>EEVRQFRRLFAQLAGDDMEVSATELMNILNKVVTRHPDLKTDGFGIDTCRSMVAVMDSDTTGKLGFEEFKYLWNNIKRWQAIYKQFDTDRSGTICSSELPGAFEAAGFHLNEHLYNMIIRRYSDESGNMDFDNFISCLVRLDAMFRAFKSLDKDGTGQIQVNIQEWLQLTMYS[2x]

Calpain-I and calpain-II are the two most studied members of a family of calcium dependent cysteine proteases that currently comprises fifteen identified gene products in humans. These heterodimeric proteases are composed of a large subunit with a molecular mass of ∼80 000 and a small subunit of mass ∼30 000. Selective inhibitors might not only be potential drugs but should act as tools to explore the physiological and pathophysiological roles of calpain-I. α-Mercaptoacrylic acid based calpain inhibitors are potent, cell permeable and selective inhibitors of calpain-I and calpain-II. These inhibitors target the calcium binding domain PEF(S) of calpain-I and -II.

The interaction of (Z)-3-(6-bromoindole-3-yl)-2-mercaptoacrylic acid with human PEF(S) was investigated by single crystal X-ray crystallography. Human PEF(S) was produced in E. coli, purified to apparent homogeneity, crystallised and soaked with 3 as previously described for other α-mercaptoacrylic acids. With the exception of a hydrogen bond between the carboxylate of 3 and the side chain amide group of Gln175 in chain B, van der Waals forces are the main interactions observed between 3 and the residues of both monomers of the protein. Based on the X-ray crystal structure of PEF(S) bound to (Z)-3-(6-bromoindol-2-yl)-2-mercaptoacrylic acid, oxidised α-mercaptoacrylic acids such as 4 were designed to target the full calpastatin binding cavity.>AVHHCKLVFFAEAAIIGLM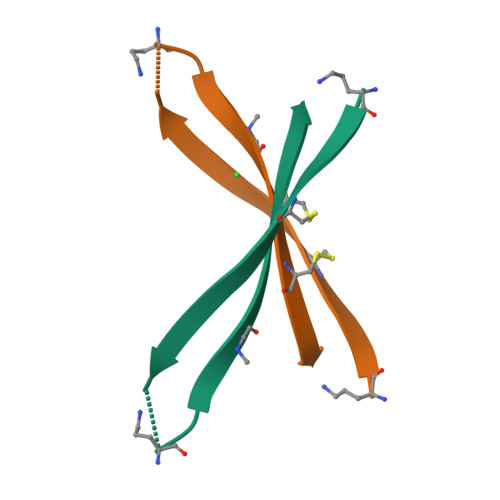VCGVV[2x]>[8x]MTPYEDLL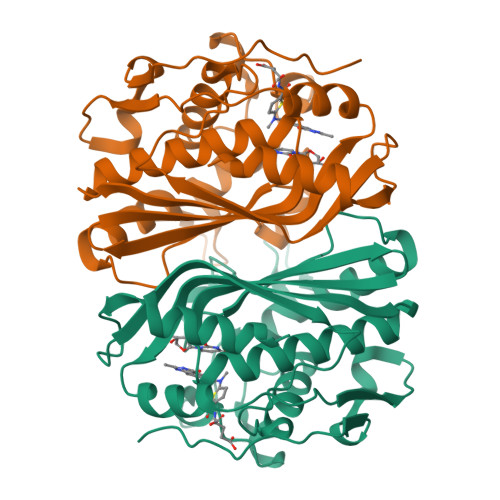RFVLETGTPKSDRTGTGTRSLFGQQMRYDLSAGFPLLTTKKVHFKSVAYELLWFLRGDSNIGWLHEHGVTIWDEWASDTGELGPIYGVQWRSWPAPSGEHIDQISAALDLLRTDPDSRRIIVSAWNVGEIERMALPPCHAFFQFYVADGRLSCQLYQRSADLFLGVPFNIASYALLTHMMAAQAGLSVGEFIWTGGDCHIYDNHVEQVRLQLSREPRPYPKLLLADRDSIFEYTYEDIVVKNYDPHPAIKAPVAV>[2x]GHMINYPLASSTWDDLEYKAIQSVLDSKMFTMGEYVKQYETQFAKTFGSKYAVMVSSGST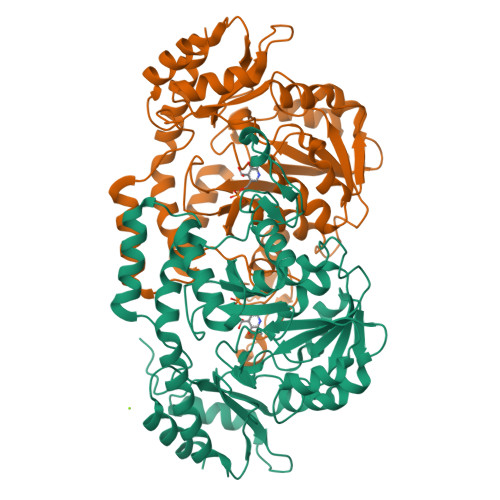ANLLMIAALFFTKKPRLKKGDEIIVPAVSWSTTYYPLQQYGLRVKFVDIDINTLNIDIESLKEAVTDSTKAILTVNLLGNPNNFDEINKIIGGRDIILLEDNCESMGATFNNKCAGTFGLMGTFSSFYSHHIATMEGGCIVTDDEEIYHILLCIRAHGWTRNLPKKNKVTGVKSDDQFEESFKFVLPGYNVRPLEMSGAIGIEQLKKLPRFISVRRKNAEYFLDKFKDHPYLDVQQETGESSWFGFSFIIKKDSGVIRKQLVENLNSAGIECRPIVTGNFLKNTDVLKYFDYTVHNNVDNAEYLDKNGLFVGNHQIELFDEIDYLREVLK>[3x]MGSMFTFL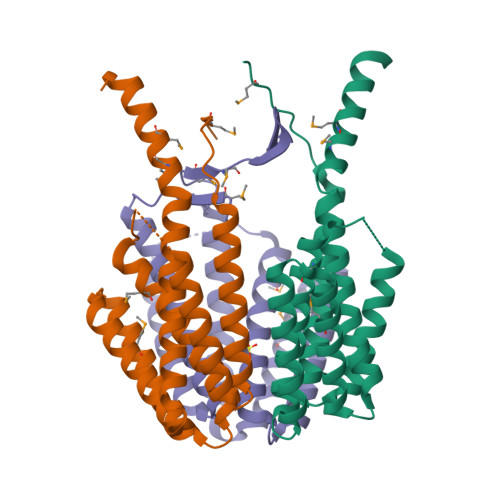LNEEETLALEQRLDTARLRADDALRFLRLGEAEEAGRIAKETSTQLRAEGQGQAPAPEVAPAASVEMTGRLDGLGRLLDAASVGYGAQSRGVLRQAVEKRVEAVTAYEKKDFAAAAAAMDGSASLLAGIAPTRTEELAGLWRLEKELATAHAAHEAARWTRPMLSMHEQLSENLYFQ> GPGYQDPNSVMTTKGHIYVIDDDAAMRD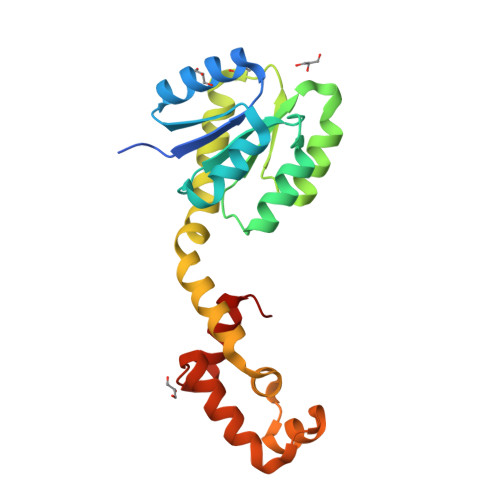SLNFLLDSAGFGVTLFDDAQAFLDALPGLSFGCVVSDVRMPGLDGIELLKRMKAQQSPFPILIMTGHGDVPLAVEAMKLGAVDFLEKPFEDDRLTAMIESAIRQAEPAAKSEAVAQDIAARVASLSPRERQVMEGLIAGLSNKLIAREYDISPRTIEVYRANVMTKMQANSLSELVRLAMRAGMLND>[2x]GAAEAGITGTWYNQLGSTFIVTAGADGALTGTYESAVGNAESRYVLTGRYDSAPATDGSGTALGWTVAWKNNYRNAHSATTWSGQYVGGAEARINTQW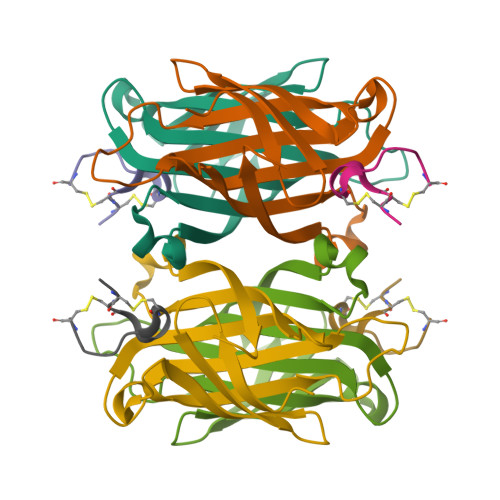LLTSGTTEANAWKSTLVGHDTFTKVKPSAAS;>RCCHPQCGMAEECR[2x]> DPSKDSKAQVSAAEAGITGTWYNQLGSTFIVTAGADGALTGTYESAVGNAESRYVLTGRYDSAPATDG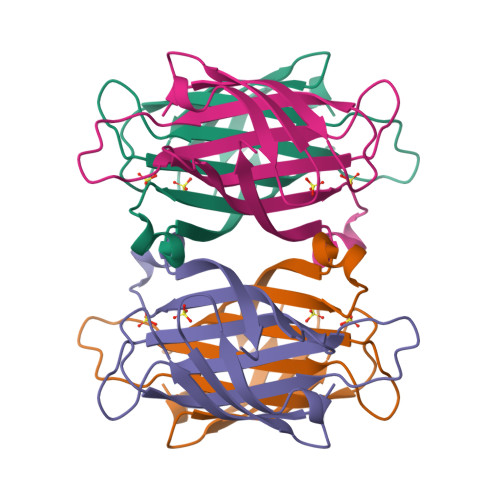SGTALGWTVAWKNNYRNAHSATTWSGQYVGGAEARINTQWLLTSGTTEANAWKSTLVGHDTFTKVKP>PREVLTGGHSVSAPQENRIYVMDSVFMHLTESRVHVYDYTNGKFLGMVPTAFNGHVQVSNDGKKIYTMTTYHERITRGKRSDVVEVWDADKLTFEKEISLPPKRVQGLNYDGLFRQTTDGKFIVLQNASPATSIGIVDVAKGDYVEDVTAAAGCWSVIPQPNRPRSFMTICGDGGLLTINLGEDGKVASQSRSKQMFSVKDDPIFIAPALDKDKAHFVSYYGNVYSADFSGDEVKVDGPWSLLNDEDKAKNWVPGGYNLVGLHR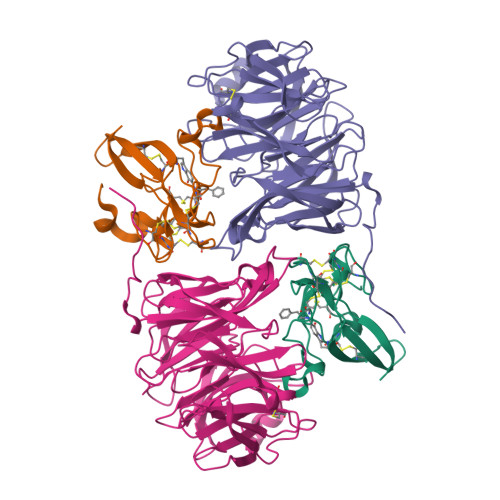ASGRMYVFMHPDGKEGTHKFPAAEIWVMDTKTKQRVARIPGRDALSMTIDQQRNLMLTLDGGNVNVYDISQPEPKLLRTIEGAAEASLQVQFHPVGGT[2x];>AGGGGSSSGADHISLNPDLANEDEVNSCDYWRHCAVDGFLCSCCGGTTTTCPPGSTPSPISWIGTCHNPHDGKDYLISYHDCCGKTACGRCQCNTQTRERPGYEFFLHNDVNWCMANENSTFHCTTSVLVGLAKN[2x]> NFGPGTELTVLPLEKTLLTESGGGTYQAGKTLSLKCQTSGFQFKTSQLDWYLWTPGHAPLWLTGLNSSSTDATEGRITSSREDNKNQIFLQIEDLGLRDSGQYHCARRVGNGDDTDKLVFGLGTRVIVEPRPAAPLSPSVFLVRDQDAVACLIRNFYPKELHVSLTSSGTLISAQSLSLAPTASGTYSAIHIGRVGENDAITCSVKHLGKEIHMSHQAGSLVPR;> ETGVALEQRPISITRNAKQSASLNCKILNPVSDYVHWYRSQEGRAPERLLVYSRSKSESVPDPGFSADKVRAYKGKDDTCRLIVSDLQVSDSGVYHCASWDGRVKVFGEGTRLIVTESAFKKKPPKPIFFLPTSEEIKQKQSGTYI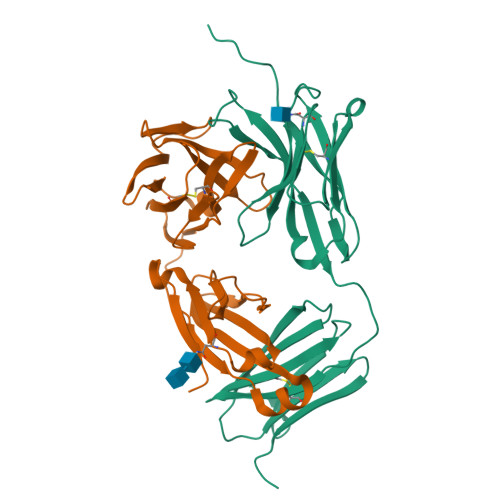CLLEDFFPNVVKTYWKEDGNSQPLDAQFGPITGGGNSYSQVSWLTVKEDVLRKNLTYFYQHEDLGMEPKAFSISSVREKGSLVPR> MATLSLTVNSGDPPLGALLAVEHVKDDVSISVE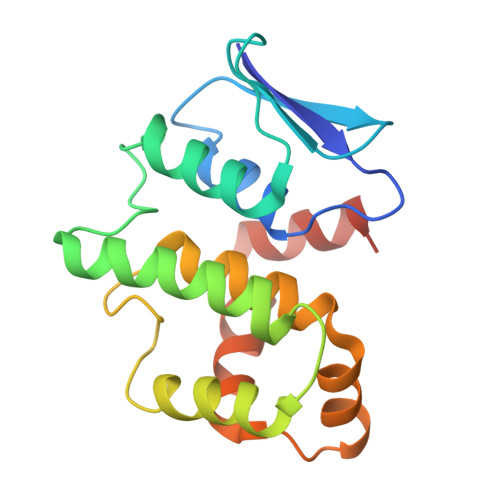EGKENILHVSENVIFTDVNSILRYLARVATTAGLYGSNLMEHTEIDHWLEFSATKLSSSDSFTSTINELNHSLSLRTYLVGNSLSLADLSVWATLKGNAAWQEQLKQKKAPVHVKRWFGFLEAQQAFQSVGTKWDVSTTKAR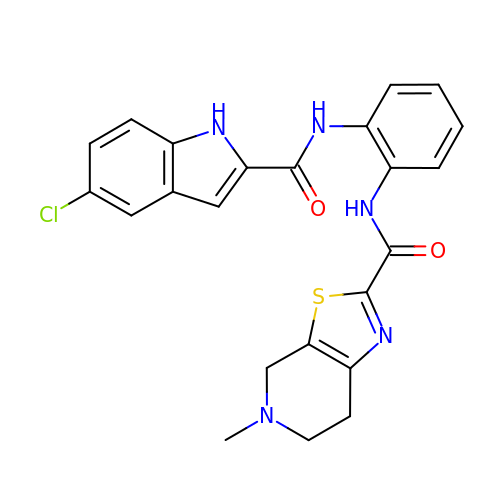N-(2-{[(5-chloro-1H-indol-2-yl)carbonyl]amino}phenyl)-5-methyl-4,5,6,7-tetrahydro[1,3]thiazolo[5,4-c]pyridine-2-carboxamide | C23 H20 Cl N5 O2 S | HLZHKMHNSZRIOD-UHFFFAOYSA-N> RVTEQMKNEADTEYYGVISIGTPPESFKVIFDTGSSNLWVSSSHCSAQACSNHNKFKPRQSSTYVETGKTVDLTYGTGGMRGILGQDTVSVGGGSDPNQELGESQTEPGPFQ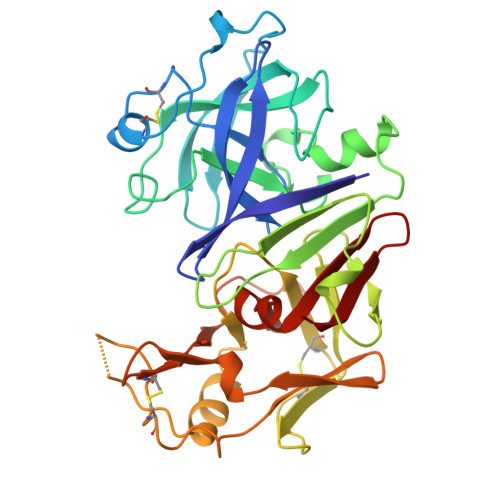AAAPFDGILGLAYPSIAAAGAVPVFDNMGSQSLVEKDLFSFYLSGGGANGSEVMLGGVDNSHYTGSIHWIPVTAEKYWQVALDGITVNGQTAACEGCQAIVDTGTSKIVAPVSALANIMKDIGASENQGEMMGNCASVQSLPDITFTINGVKQPLPPSAYIEGDQAFCTSGLGSSGVPSNTSELWIFGDVFLRNYYTIYDRTNNKVGFAPAA> MGSSHHHHHHSSGLVPRGSHMAAAPEAVTAADPEDAAFWTAVEDGDVSALTAALGTDEDSVAAVLPALSSWRRARKERSTVDSWRYRPTWKPVTKLPQRTLDGTWLLVSADGVDDTDVAEALETGGAEVRRLVLDESCTDRAVLRERLTDADGLTGIVSVLAGAERTGAVPGTGLVLGVALTVALVQALGDAGIDTPLWALTRGAVSTGRSDKVTAPVQAQVTGIGWTAALECPGRWGGVVDLPETLDARAGQRLAAVLAGALGDDDQIALRSSGVFTRRIVRADAAPDGSARDWKPRGTTLVTGGSGTLAPHLARWLAEQGAEHLVLVSRRGPEAPGAAELRAELAERGTETTLAA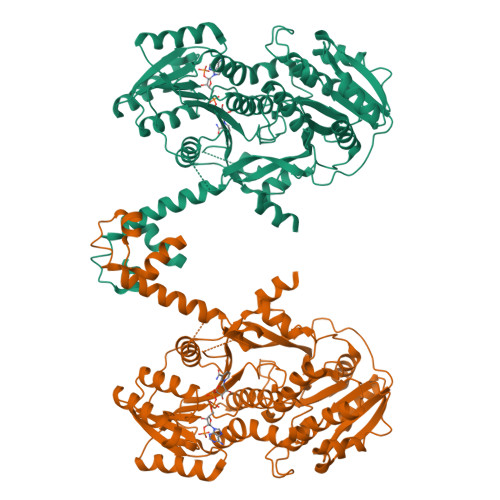CDITDRDAVAALLESLKAEGRTVRTVVHTAATIELHTLDATTLDDFDRVLAAKVTGAQILDELLDDEELDDFVLYSSTAGMWGSGAHAAYVAGNAYLAALAEHRRARGLTALSLSWGIWADDLQLGRVDPQMIRRSGLEFMDPQLALSGLKRALDDDEQVIAVADVDWETYHPVYTSARPTPLFDEVPEVQRLTAAAEQSAGDPARGEFAAALLALPAAEQHR>[2x]MSSKEELAPKLESIMSEISVCEGLVLAKNNGDVLIGQ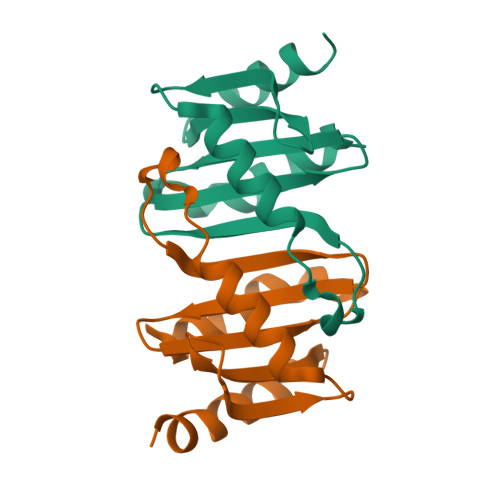TLTEMDHNSIAKSVSKMFKTKIDALNKGNLLEMTLGMDEGFLIAVKNNDLMVLGFLGPDGRSSVGLLLRQLKNIMK(6R)-1,6-anhydro-2-O-heptyl-6-(hydroxymethyl)-D-galactitol 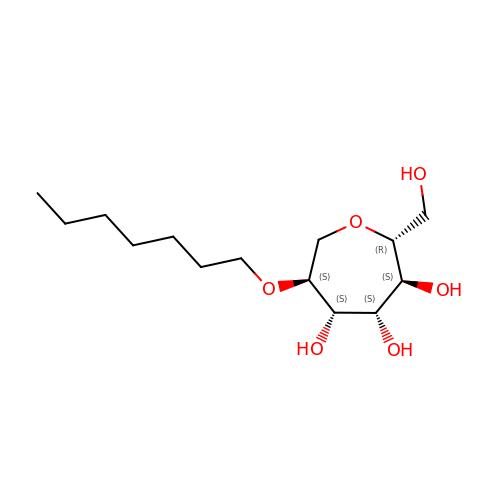| C14 H28 O6 | WXAPBESCSQWOGD-ITGHMWBKSA-N>MKSSHHHHHHENLYFQSNATKKSAAEASKKPRQKRTATKAYNVTQAFGRRG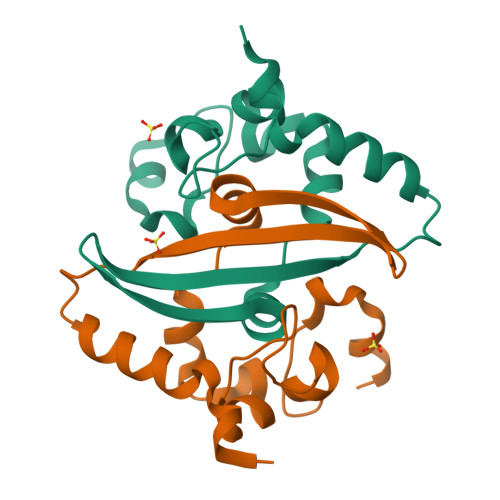PEQTQGNFGDQELIRQGTDYKHWPQIAQFAPSASAFFGMSRIGMEVTPSGTWLTYTGAIKLDDKDPNFKDQVILLNKHIDAYKTFP[4x]> EVEEF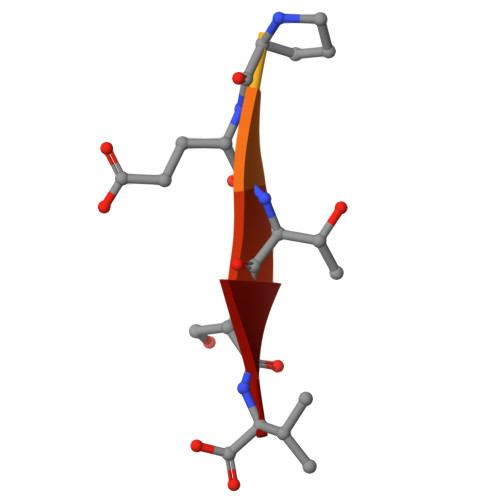PETSV Members of GH family 73 (GH73) are β-N-acetylglucosaminidases that cleave the β-1,4 glycosidic linkage between the N-acetylglucosamine (GlcNAc) and N-acetylmuramic acid (MurNAc) residues of bacterial cell wall peptidoglycan (PG). In some instances, GH73 enzymes are associated with bacterial pathogenicity, for example, LytB being critical for pneumococcal nasal colonization and cell division, Auto for pathogenic listeriosis caused by Listeria monocytogenes, and FlgJ for biogenesis and function of the flagellum, which is a major virulence factor of motile pathogenic bacteria. The domain was found to adopt a lysozyme-like fold common to other GH73 enzymes, which consists of an α-helical subdomain packed against a β-lobe that forms an extended β-hairpin motif. The α-helical domain and β-hairpin of StFlgJGH(151–316) together form a groove-shaped active site, with the α-helical subdomain containing an α-central helix that houses a conserved glutamate general acid/base (E184), and the β-hairpin, in turn, containing a second glutamate residue (E223) previously determined to be required for GH activity.

To explore the structural basis of FlgJ activity, we determined the crystal structure of the FlgJ GH domain from S. typhimurium (StFlgJ) to 1.8 Å resolution. Interestingly, the active site of StFlgJGH(151–316) was found to be occupied by the C-terminal α-helix of a neighbouring symmetry mate. The C-terminal α-helix StFlgJGH(151–316) packs into the active site of the symmetry mate via hydrophobic and hydrogen-bonding interactions. Hydrophobic interactions were found to occur between L312 of the helix and F204 and Y249 of the active site of the symmetry mate, as well as between Y308 of the helix and L183 and Y286 of the symmetry mate active site. Hydrogen bonds occur between Y308 and N311 of the helix and K289 and backbone amide of Y280 of the symmetry mate active site. Residues 223–229—which form a loop connecting the two strands of the β-hairpin motif—were disordered and could not be modeled. Similar results have been reported for the crystal structures of other GH73 enzymes, indicating that the β-hairpin is likely mobile in this family of enzymes. A superposition of the StFlgJ and SpFlgJ GH domain structures with Auto reveals that the C- and N-termini of these enzymes are spatially conserved, which suggested that FlgJ might be auto-inhibited by the C-terminal α-helix, in similar fashion to the auto-inhibition of Auto by an N-terminal α-helix. To determine whether the C-terminus of StFlgJGH(151–316) autoinhibits the enzyme in solution, the full-length StFlgJ GH domain, StFlgJGH(151–316) and a C-terminal truncated form of the domain (StFlgJGH(151–301)) were tested for activity using a zymogram assay. Contrary to our hypothesis, we found the catalytic activity of StFlgJ to be unaffected by presence or absence of its C-terminal α-helix, suggesting the helix does not regulate function.

> MDSKDFLARLSLPARLASEQSGVPHHLILAQAALESGWGQRQILRENGEPSYNVFGVKATASWKGPVTEITTTEYENGEAKKVKAKFRVYSSYLEALSDYVALLTRNPRYAAVTTAATAEQGAVALQNAGYATDPNYARKLTSMIQQLKAMSEKVSKTYSANLDNLFGSHHHHHH>MSEMTPREIVSELDKHIIGQDNAKRSVAIALRNRWRRMQLNEELRHEVTPKNILMIGPTGVGKTEIARRLAKLANAPFIKVEATKFTEVGYVGKEVDSIIRDLTDAAVKMVRVQAIEKNRYRAEELAEERILDVLIPPAKNNWGQTEQQQEPSAARQAFRKKLREGQLDDKEIEIDLAAAPMGVEIMAPPGMEEMTSQLQS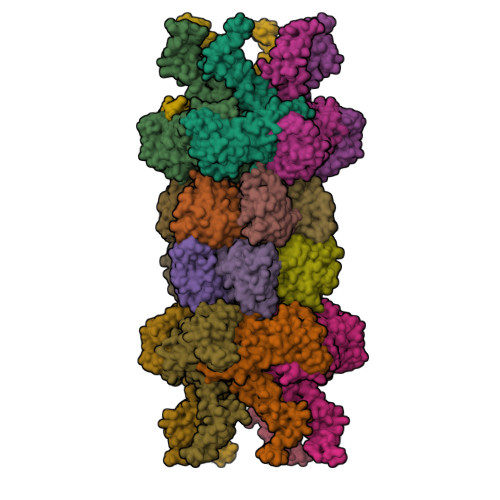MFQNLGGQKQKARKLKIKDAMKLLIEEEAAKLVNPEELKQDAIDAVEQHGIVFIDEIDKICKRGESSGPDVSREGVQRDLLPLVEGCTVSTKHGMVKTDHILFIASGAFQIAKPSDLIPELQGRLPIRVELQALTTSDFERILTEPNASITVQYKALMATEGVNIEFTDSGIKRIAEAAWQVNESTENIGARRLHTVLERLMEEISYDASDLSGQNITIDADYVSKHLDALVADEDLSRFIL[4x];>[4x]TTIVSVRRNGHVVIAGDGQATLGNTVMKGNVKKVRRLYNDKVIAGFAGGTADAFTLFELFERKLEMHQGHLVKAAVELAKDWRTDRMLRKLEALLAVADETASLIITGNGDVVQPENDLIAIGSGGPYAQAAARALLENTELSAREIAEKALDIAGDICIYTNHFHTIEELSYKA>[2x]SMHAIEVTETGGPGVLRHVDQPQPQPGHGELLIKAEAIGVNFIDTYFRSGQYPRELPFVIGSEVCGTVEAVGPGVTAADTAISVGDRVVSASANGAYAEFCTAPASLTAKVPDDVTSEVAASALLKGLTAHYLLKSVYPVKRGDTVLVHAGAGGVGLILTQWATHLGVRVITTVSTAEKAKLSKDAGA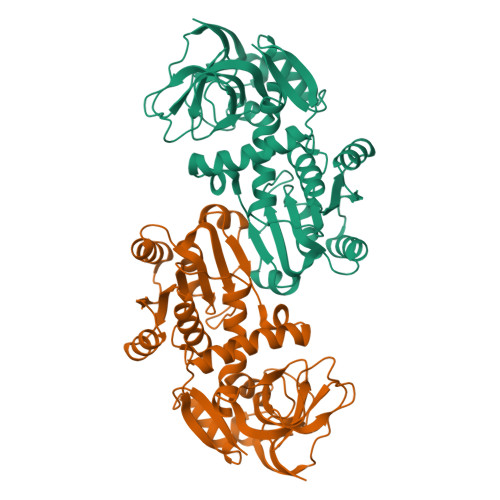DVVLDYPEDAWQFAGRVRELTGGTGVQAVYDGVGATTFDASLASLAVRGTLALFGAASGPVPPVDPQRLNAAGSVYLTRPSLFHFTRTGEEFSWRAAELFDAIGNEAITVAVGGRYPLADALRAHQDLEARKTVGSVVLLP>[2x]MGLEKTVKEKLSFEGVGIHTGEYSKLIIHPEKEGTGIRFFKNGVYIPARHEFVVHTNHSTDLGFKGQRIKTVEHILSVLHLLEITNVTIEVIGNEIPILDGSGWEFYEAIRKNILNQNREIDYFVVEEPIIVEDEGRLIKAEPSDTLEVTYEGEFKNFLGRQKFTFVEGNE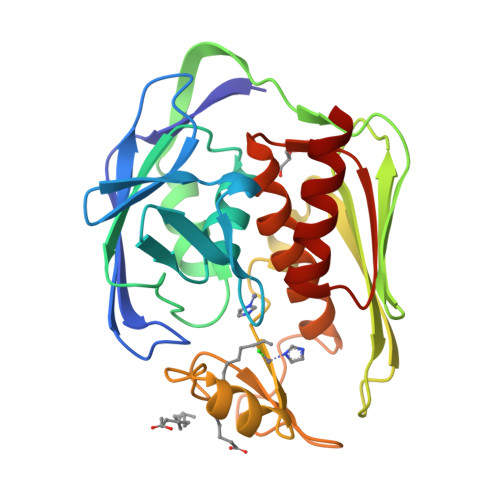EEIVLARTFAFDWEIEHIKKVGLGKGGSLKNTLVLGKDKVYNPEGLRYENEPVRHKVFDLIGDLYLLGSPVKGKFYSFRGGHSLNVKLVKELAKKQ Here, we explain the mechanism by which the phage AR9 non-virion RNAP (nvRNAP), a bacterial RNAP homolog, recognizes the −10 element of its deoxyuridine-containing promoter in the template strand. The AR9 sigma-like subunit, the nvRNAP enzyme core, and the template strand together form two nucleotide base-accepting pockets whose shapes dictate the requirement for the conserved deoxyuridines. The catalytically active AR9 nvRNAP core enzyme consists of four proteins that, when pairwise concatenated, show about 20% sequence identity and cover the entire lengths of the universally conserved β and β′ subunits of bacterial RNAPs. Promoter-specific transcription is performed by a five-subunit holoenzyme that, in addition to the nvRNAP core, contains the product of AR9 gene 226 (gp226).

We have crystallized the AR9 nvRNAP core in two different crystal forms that had a “Standard” and “Large” unit cell containing two and eight nvRNAP core molecules in the asymmetric unit, respectively. The Standard and Large unit cell crystals diffracted X-rays to 3.30 Å and 3.79 Å resolutions, respectively. The electron density in all datasets was poor and displayed a large amount of disorder, which complicated the process of atomic model building. The X-ray structure of the core will be referred to as AR9 nvRNAP-core-Xray. In the AR9 nvRNAP-core-Xray structure the TLID has located roughly in-between the β and β′ pincers where it partially obstructs the downstream DNA channel. The TLID carries a negative charge on its DNA-facing surface. Similar to the negatively charged σ1.1 domain of bacterial σ70 factors, the AR9 nvRNAP TLID may function to inhibit non-specific interactions of the enzyme with nucleotide templates. Out of 10 independent copies of the AR9 nvRNAP core belonging to two different crystal forms of AR9 nvRNAP-core-Xray datasets (Standard and Large unit cell crystals), the TLID is ordered in only one molecule.

>[2x]MDDISVIKNEDYEGSHRFLAEELLMPNANKTDGNRSTMFCSHLAQAVTLQKAEPPLVYTNFENQVGKYSTAGYRKANSNYKVIEKIYKNDYNYVLIVQDQETGEYTLFERAECEFLTEHYGFQWDNDKIDSLKKDDTIEKDTVLYKNTCYDENMNFGYGVNLNAAYFSYKNETLEDAIVISESAAKKLGTFSVNKVKVSVNTNDILLNLYGDNENYKGFPDIGEHIKNQIIASRRRFDYNTALYELKNLNEMRDSDTPFFADGKIVDIEIFSNVPEEELKVQKYNEQVLYYINKQKEFSNNVYQKLKKIVEGKDNNVSDKLLHFYNNCKMRIDENISYTYQNSKFSGFIMEFTILEEEPLNKGSKITGRYGNKGVISKILPDDQMPTVAEGRFKGLKADICLNPLGVFNRLNPSQLIEQELNWIAKFIRKDMEEAGSNEEKVSILLDFLNRVNKEETELMEEFINSLNKTELEEFLNDIIENGIPICQKPFFGNIGLDELWELYNHYDHIDYFKCEGISTPLIIGEIYMVRLKHEPHSKFSARSTSFMNLRGLPAKSKNFKEHKDLYSKTPVRIGNMEISNLSLTNEMGSIMDMLNSYSNNETNRRELIMQLLTGNPFDTNIDLSDVESGTSKILKSLFTCLGLSIDDVEEEWENKLNGKVEDEK;>MEKTYNLNDILLSNEYEKIKEDIKEEIINDMASKKVKYSNTSEFAKNDFLKDEFIDLVVDGETYEITYGNLITLLIVARPFNHFKVPMTEDLLFDLSDLKEYQNYYTTLLEHFGYSNEIKSIIKDVISELAIFSGDINVTFGNTVSIKSLIDLGNKVKRFRELLHYRLPNDEALEFNDIEAIIKKNLDEIMKILSETDNMLRYYIDSGAGINSKQFGQVLSLVGSKPDLFGKIIPYPINTSFLRGLDVRSFYINALGARKALITNYQQVRNSGYLTRKISMLLMDTKLIDLDDCGSHENNYLSINVENKDVLKRFSKRSYLNNNGELVEIDINDESLIGQVIKIPSPTTCASNEGVCRKCYGKLFDINKDLNIGMIAVLLLTDPLTQRLLSAKHLLETRSSKIDWGTNFEENFIVNRNLIYPKVYNGTVIIKEDDFKEDEETEEQVFDTFTLKSGNRFISISSPMRLFLNKDLKKQLDESFYNIEEMQFEIPLNKLDEGDSFATFIMDNNELSKPLREIKDLIETNKYIKDHNVNEVVNYFIYLLNESGINIQSVHSELIIREMMKLDDSDRTQFKNDKMPDYEIFRITDANLKGDSLSRSLLFEQVKKQLTTLDYDTFNKTKSSILDKLL[2x];>[2x]MISNFRKFHGNKNQEKFNENLILNKENESILNYLDPICKTLEIIPEITYLGSSVEPINKVYKFNKEEKTSDIERSELQLIKMSFLIEKDDKKEEINKFIYFPKLIDSQYFIINGNRYYPIYQLLDSGTYRTNKALTLKTLLMPIVLREKKETFDDINGETHTMLNVDLDLFKSKVPFLIYFFSKFGFEGTLEYFGLQDLIHVLMKEDLDQLDEDEINDNVIFMITKNISLVVDKNFFSNKNNQIIIATLLNCFNTRIKIDKIYEKDYWVKKLGGYFTTNNSNKQEKGEGIILSFERILDEWTKKILRTEEKNKEDIYSVVRWMINNYLALVKQDNMNLANKRIRLYEYLLHPLLIKFSKGTYRVLNNRNSNKFEKIKTIFSNIQEGFLVKKIINNELLRYDNSVNSISLFTLILRYTQSGPQSPFSSNSTNNKLRGLHPSYLGRLGLTSTSAGDPGASGSLTPFLELPENSYMHFTEEPEINLNIDDISIDEVIES;>[2x]MGSSHHHHHHSSGENLYFQGHHMGKKLSLIDFNEIYNEENLITRANPIENHEFSDDGIYSERIFGSYNEDDDDKDIDTIGWINIEPYYIINPILFTIIKKCIPSINKIINYQQSIDQNGENIDLTEEIGEDDYIGLVKFKDNFDDLLEKYTDKKKYQKEYDFLIENHDKIFINKLPVFSHKLRPATLLTGSKGKVLAFDEINNYYNFVIEYINQINEGVVSDDSIDLLLLPLLYNMQFYANNILTRIISEYLRGKKGFLRKNIMGSRINFSARNVITPLIGHPIDEVAMPYKTFAELYKFQLINLISKVKGINYNEALKFWEKGILGFNQELYNYMEELITKTKGGCTFLLNRNPTISIGSILYLKIGLIKKDYKDLTLGISNNLLSALSGDYDGDVLNIIPVFDNKMKEHFSLLSPQNFLVDRNNGRFNGDFDLQKDQILGIFILNN>[4x]MGRKKIQITRIMDERNRQVTFTKRKFGLMKKAYELSVLC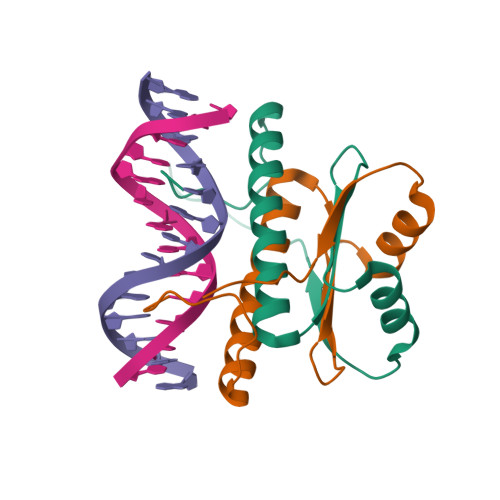DCEIALIIFNSSNKLFQYASTDMDKVLLKYTEYSEPHESRTNTVILETLKRREHRG>[2x]MVKSSGTERKE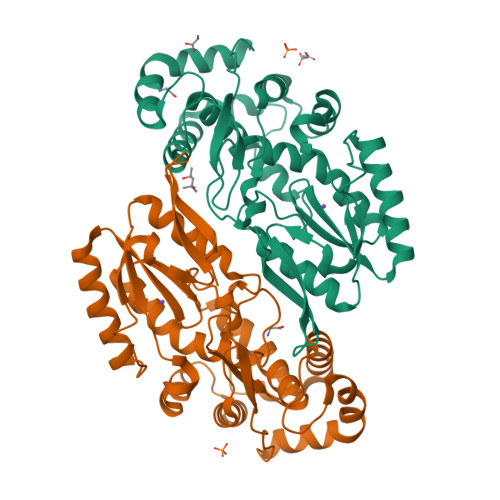RMDTSSLMEQILSNDNLNRAYLQVVRNKGAEGVDGMKYTELKEYLAKNGEIIKEQLRIRKYKPQPVRRVEIPKPDGGVRNLGVPTVTDRFIQQAIAQVLTPIYEEQFHDHSYGFRPNRCAQQAILTALDMMNDGNDWIVDIDLEKFFDTVNHDKLMTIIGRTIKDGDVISIVRKYLVSGIMIDDEYEDSIVGTPQGGNLSPLLANIMLNELDKEMEKRGLNFVRYADDCIIMVGSEMSANRVMRNISRFIEEKLGLKVNMTKSKVDRPRGIKYLGFGFYYDTSAQQFKAKPHAK> GAMGMTTDEGAKNNEESPTATVAEQGEDITSKKDR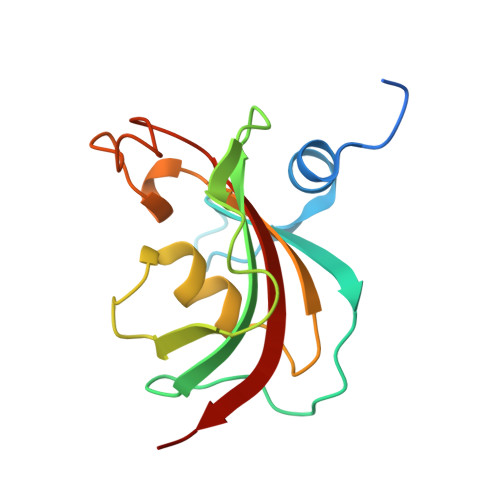GVLKIVKRVGNGEETPMIGDKVYVHYKGKLSNGKKFDSSHDRNEPFVFSLGKGQVIKAWDIGVATMKKGEICHLLCKPEYAYGSAGSLPKIPSNATLFFEIELLDFKGE ADENINE 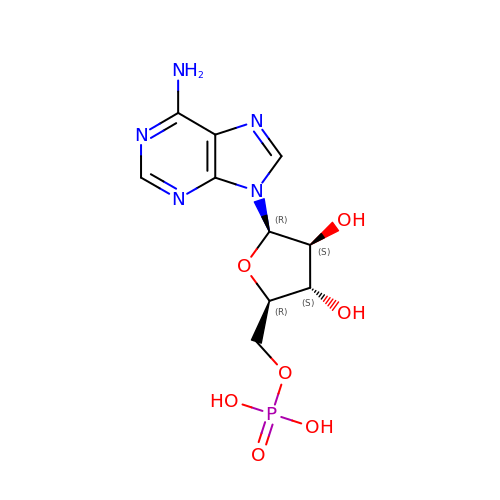ARABINOSE-5'-PHOSPHATE | C10 H14 N5 O7 P | UDMBCSSLTHHNCD-UHTZMRCNSA-N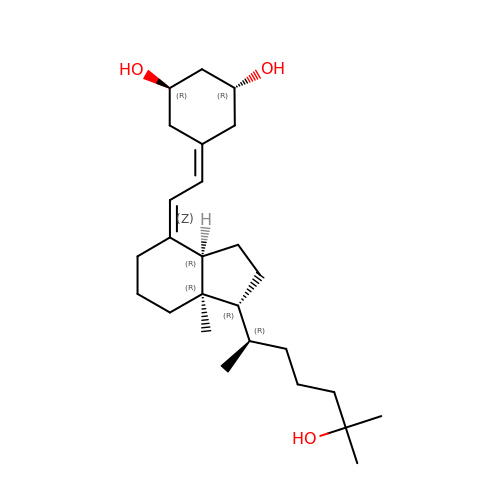(1R,3R,7Z,14beta,17alpha)-17-[(2R)-6-hydroxy-6-methylheptan-2-yl]-9,10-secoestra-5,7-diene-1,3-diol | C26 H44 O3 | PKFBWEUIKKCWEW-VWYYVUTKSA-N> MAPWKIEEVKTLKGLIKSKPVVAIVDMMDVPAPQLQEIRDKIRD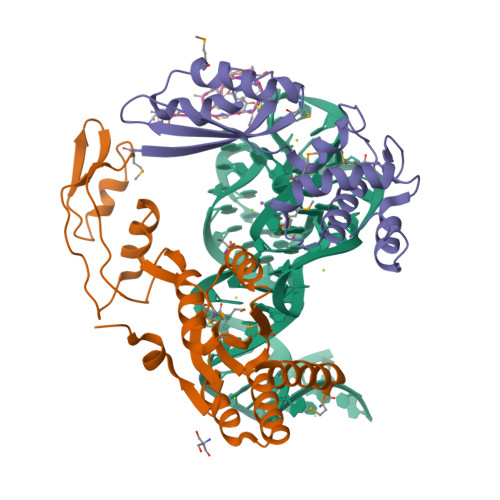KVKLRMSRNTLIIRALKEAAEELNNPKLAELANYVERGAAILVTDMNPFKLYKLLEENKSPAPVRGGQIAPCDIKVEKGSTGMPPGPFLGELKSVGIPAAIEKGKIAIKEDKVVVKKGEVVSPKLAAVLDRLGIKPIKVGLNILAVYEDGIIYTPDVLKVDEEKLLADI;> MAKEVVEVLVTGGRATAGPPLGPAIGPLGVNVMQVVKEINEKTKDYEGMQVPVKVIVDTETRKFEIEVGIPPTTALIKKELGIETAAHEPRHEVVGNLTLEQVIKIAKMKKDAMLSYTLKNAVKEVLGTCGSMGVTVEGKDPKEVQKEIDAGVYDEYFKEE;> XIASASCTTCICTCSCSSX> SS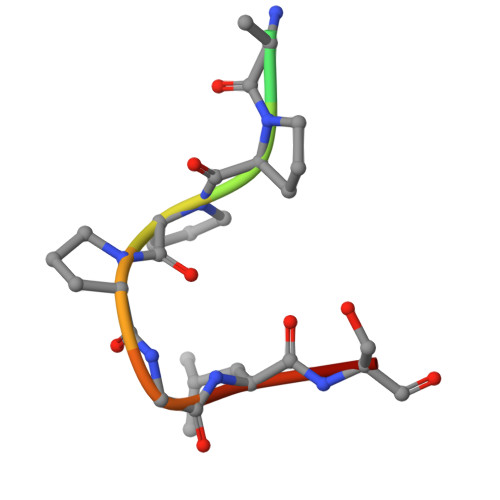IAPPPGLSG>KDGDQCETSPCQNQGKCKDGLGEYTCTCLEGFEGKNCELFTRKLCSLDNGDCDQFCHEEQNSVVCSCARGYTLADNGKACIPTGPYPCGKQTLER[2x];>IVGGQECKDGECPWQALLINEENEGFCGGTILSEFYILTAAHCLYQAKRFKVRVGDRNTEQEEGGEAVHEVEVVIKHNRFTKETYDFDIAVLRLKTPITFRMNVAPACLPERDWAESTLMTQKTGIVSGFGRTHEKGRQSTRLKMLEVPYVDRNSCKLSSSFIITQNMFCAGYDTKQEDACQGDSGGPHVTRFKDTYFVTGIVSWGEG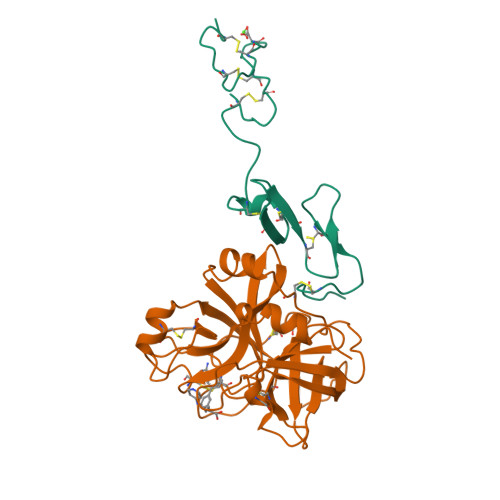CARKGKYGIYTKVTAFLKWIDRSMKTR[2x]Roquins are a family of RNA-binding proteins critically involved in maintaining peripheral immunological tolerance and preventing autoimmune diseases. The human genome encodes two Roquin paralogs, RC3H1 and RC3H2. The N-terminal regions of these two proteins are highly homologous and are composed of a RING (Really Interesting New Gene)-type E3 ubiquitin ligase domain, followed by a unique, so-called ROQ domain of approximately 300 amino acid residues and a CCCH-type ZnF domain5. The ROQ domain binds to a highly conserved, stem-loop-forming constitutive decay element (CDE), which is found in the 3′ UTR of many mRNAs encoding regulators of development and inflammation.

We next determined the crystal structure of RC3H2 in complex with a 15-nt constitutive decay element (CDE) of human intermediate early response 3 (Ier3) RNA at 2.5 Å resolution. Surprisingly, each asymmetric unit (ASU) contains two protein molecules, two single-stranded RNAs, and one double-stranded (ds) RNA. The single-stranded RNA binds to the winged helix-turn-helix (wHTH)-like region23 of the ROQ domain, similar to previously reported RC3H1 structures in complex with different CDE RNAs212223, while the RNA duplex binds to the HEPN and ROQ domains simultaneously. The single-stranded Ier3 RNA forms a stem-loop structure containing five Watson-Crick base pairs and a UGU trinucleotide loop. The stem-loop RNA interacts with the ROQ domain mainly using most of the phosphate groups in the 5′ arm and the trinucleotide loop, while the 3′ half of the stem does not form direct interaction with the protein. A detailed crystallographic analysis suggests that the two RC3H2 molecules in the ASU bind to the RNA duplex in a similar but not identical way. Both protein molecules use residues in the ROQ domain to interact with the backbone of one RNA strand (chain C), while residues in the HEPN domain interact with the backbone of the other RNA strand (chain D). Notably, side chains of Ser312, Gln315, and Asp319 of both protein molecules form hydrogen bonds with the hydroxyl group on the pentose ring of two adjacent ribonucleotides, suggesting an RNA- but not DNA-specific interaction. The most distinctive feature is the interaction between the guanidinium group of the Arg128 side chain from the HEPN domain of protein molecule A with the purine base of the central G8 from RNA chain D. In contrast, the two RC3H2 molecules in the Ier3 complex bind to the dsRNA in a head-to-toe mode, and the two protein molecules do not interact. Indeed, when RC3H2 binds to the dsRNA, the ROQ domain rotates 42° along an axis intersecting the HEPN and ROQ domains to accommodate the interactions.

>[2x]GSNLGENKHYEVAKKCVEDLALYLKPLSGGKGVASLNQSALSRPMQRKLVTLVNCQLVEEEGRVRAMRAARSLGERTVTELILQHQNPQQLSANLWAAVRARGCQFLGPAMQEEALKLVLLALEDGSALSRKVLVLFVVQRLEPRFPQASKTSIGHVVQLLYRASCFKVTKRDEDSSLMQLKEEFRSYEALRREHDAQIVHIAMEAGLRISPEQWSSLLYGDLAHKSHMQSIIDKLQSPESFAKSVQELTIVLQRTGDPANLNRLRPHLELLANIDPNPDAVSPTWEQLENAMVAVKTVVHGLVDFIQNYSRKGHETPQ> MGFTRLLTLVVTVASLLRFDQVTGAHTNDIRSLRARQDTAVPVYDTCTVPGSFALTFDDGPYGFSTRLDSTLNAANAKGSFFINGQNWGCIYDYADVLLERFNNGHFIASHTWSHVHMNQGTYEQLSHQLELVEQAMIRILGVKPLYMRPPYGEYNDVVLQVLRDRGYKGLIMWNQDSGDTFTPTPSSAQIIDSYRSFPEKTISLNHEIKDFTVDQVIPAVIPILQQKGFSLQTVPECLGLSSDPADWYVRVQEPGTRDDSWTCEATPLPGNFEHHHHHH

Phytopathogenic fungi secrete chitin deacetylase (CDA) to escape the host’s immunological defense during infection. Five crystal structures of two representative and phylogenetically distant phytopathogenic fungal CDAs, VdPDA1 from Verticillium dahliae and Pst_13661 from Puccinia striiformis f. sp. tritici, were obtained in ligand-free and inhibitor-bound forms. These structures suggested that both CDAs have an identical substrate-binding pocket and an Asp-His-His triad for coordinating a transition metal ion. Our findings revealed that phytopathogenic fungal CDAs share common structural features, and provided BHA as a lead compound for the design of CDA inhibitors aimed at attenuating crop fungal diseases.

Xu et al. reported that the wheat leaf-infecting pathogen Puccinia striiformis f. sp. tritici secretes a CDA (Pst_13661) during the early stages of infection. As the crystal structures revealed that Zn2+ was coordinated by the Asp-His-His triad, we considered metal ion chelators, specifically BHA and its derivatives, as potential inhibitors of CDA. To prove that BHA functioned as a metal ion chelator of CDAs, the crystal structures of Pst_13661 in complex with BHA and compounds 2 and 3 were resolved. BHA chelates a zinc ion in bidentate mode. The hydroxamic acid moiety of BHA forms three hydrogen bond interactions with the enzyme: (i) its C = O with the NH backbone of Tyr152, (ii) its NH with the imidazole group of catalytic His207, and (iii) its OH with the carboxylic acid group of Asp58. The benzene ring moiety of BHA fits a cavity formed by the nonpolar residue Leu205 and the aromatic residues Tyr152 and Trp174. The crystal structures of Pst_13661 complexed with BHA or its derivatives suggest that BHA inhibits the activity of Pst_13661 by binding to the zinc ion. We obtained benzohydroxamic acid (BHA), a lead compound, by structure-guided screening, which showed high activity against diseases in cotton, wheat, and soybean caused by V. dahliae and four other top 10 fungal plant pathogens for molecular plant pathology, namely P. striiformis f. sp. tritici, F. oxysporum, Fusarium graminearum, and Rhizoctonia solani.INDOLINE | C8 H9 N | 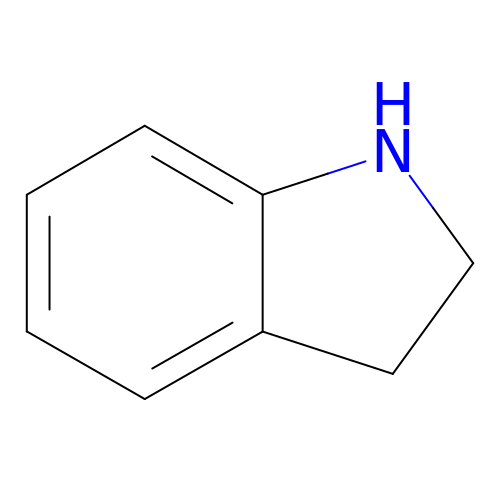LPAGFVYQRIESJQ-UHFFFAOYSA-N> SSKKRCFKRS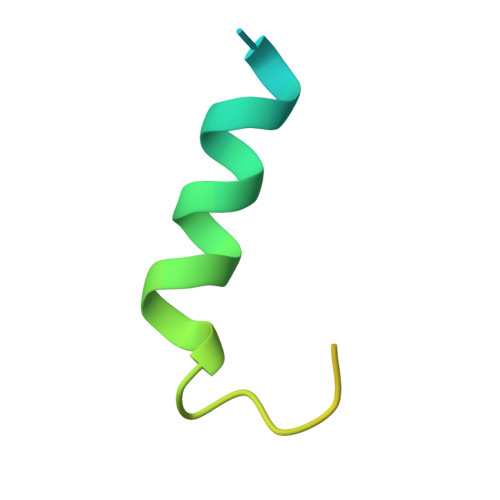SSTSKLLNKVAARASSMGTILGASIEGTLISSTPLSSCL>[10x]PVDVSVSIFINKIYGVNTLEQTYKVDGYIVAQWTGKPRKTPGDKPLIVENTQIERWINNGLWVPALEFINVVGSPDTGNKRLMLFPDGRVIYNARFLGSFSNDMDFRLFPFDRQQFVLELEPFSYNNQQLRFSDIQVYTENADNEEIDEWWIRGKASTHISDIRYDHLSSVQPNQNEFSRITVRIDAVRNPSYYLWSFILPLGLIIAASWS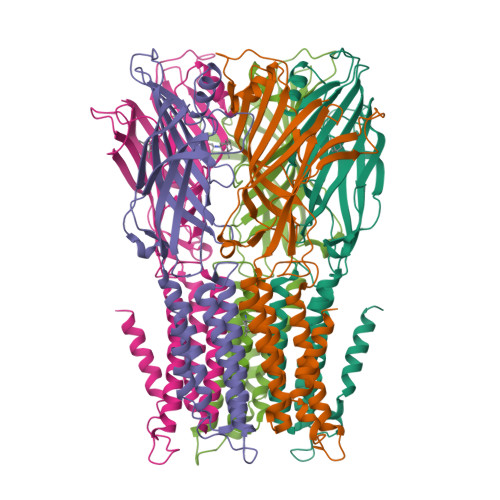VFWLESFSERLQTSFTLMLTVVAYASYTSNILPRLPYTTVIDQMIIAGYGSIFAAILLIIFAHHRQANGVEDDLLIQRCRLAFPLGFLAIGCVLVI>MSKTIKVALAGAGAFGIKHLDGIKNIDGVEVVSLVGRRFDQTKEVADKYGIAHVATDLAESLALPEVDAVILCTPTQMHAEQAIACMKAGKHVQVEIPLADALKDAQEVAELQKQTGLVAMVGHTRRFNPSHQWVHKKIEAGEFNIQQMDVQTYFFRRTNMNALGQARSWTDHLLWHHAAHTVDLFAYQAGSPIVKANAVQGPIHKDLGIAMDMSIQLKAANGAICTLSLSFNNDGPLGTFFRYIGDTGTYLARYDDLYTGKDEKIDVSQVDVSMNGIELQDREFFAAIREGREPNSSVQQVFNCYKVLHDLEQQLNAD[6x]

The key enzyme in the microbial production of PDC is 4-carboxy-2-hydroxymuconate-6-semialdehyde (CHMS) dehydrogenase, which acts on the substrate CHMS. CHMS dehydrogenase, on the other hand, has only been characterized functionally from Sphingomonas SYK-6 (10) and Pseudomonas ochracea. These studies have demonstrated that the enzyme is a NADP+/NAD+-dependent oxidoreductase with a cofactor preference for NADP+. By sequence analysis using Interpro, PmdC is classified under the Rossmann fold-NAD(P)+ binding oxidoreductase superfamily, sharing common structural characteristics with the Gfo/Idh/MocA oxidoreductase protein family.

The crystal structure of PmdC bound to NADP was solved to a resolution of 2.34 Å, spanning 98.75% of the protein sequence, Lys 3–Asn 317. Each asymmetric unit contained six copies of PmdC, existing as three dimers. The crystal structure revealed dimerization occurs at the interface between the C-terminal ß-sheets of each monomer. Each monomer has two domains: An N-terminal cofactor-binding domain bound to NADP (residues 1–141) and a C-terminal substrate binding and oligomerization domain (residues 145–317). NADP is bound to PmdC within a tube-like cavity formed at the interface between the N-and C-terminal domains. Residues within this sequence participate in stabilization of the diphosphate backbone of NADP. This includes hydrogen bond and electrostatic interactions between the main-chain peptide backbone of Ala12, Gly13, and Ala14 with the diphosphate group of NADP. Structural data revealed density within this region that was best fit with a sulfate ion from within the crystallization solution. The His177A mutant exhibited a 98% loss of activity while the H178A and H181A mutants showed an 89% and 83% loss of activity respectively compared to WT PmdC.(6R)-2-amino-4-oxo-3,4,5,6,7,8-hexahydropteridine-6-carboxylic 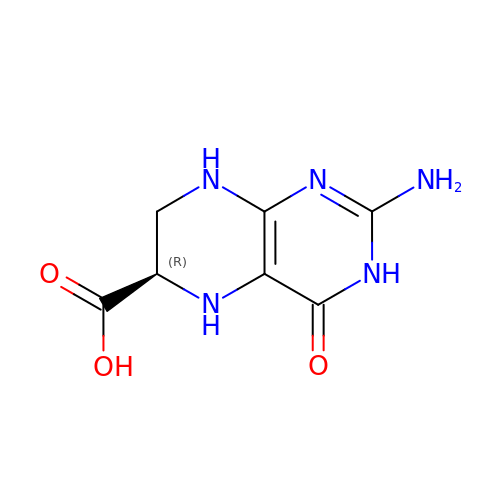acid | C7 H9 N5 O3 | QSIYONWVWDSRRO-UWTATZPHSA-N> DTGERRCDPIRISMCQNLGYNVTKMPNLVGHELQTDAELQLTTFTPLIQYGC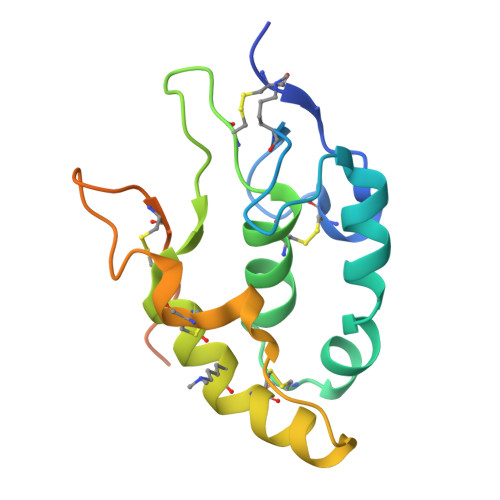SSQLQFFLCSVYVPMCTEKINIPIGPCGGMCLSVKRRCEPVLKEFGFAWPESLNCSKFPPQNDHNHMCMEGPGDEEVPLPHKTPIQPGEGTLEVLFQ> ARSYGNGVYCNNKKCWVNRGEATQSIIGGMISGWAS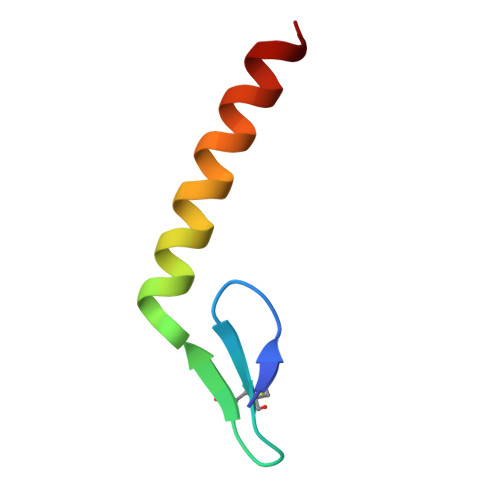GLAGM> AMSEAYNWKSVVTGAGGGFVPGIIFNQSEPDLIYARTDIGGAYRWNQATGSWVSISDAVGWVDWNKNGVDALATDPVDPDKVYMATGTYTNSWDDNGQIMRSGDRGNTWQSTPLPFKVGGNMPGRSAGERLVIDPNKNSILFFGARSGNGLWKSTDSGVTWSKVSSFPNVGTYIQNPTLEYGNDLVGLSWITFDPNTGTPGNATQTIYVGVADTASSVYRSTDGGATWTAIPGQPTGYLPHHGVLSSTGDLYITYSNGVGPYDGSKGEVWKLNTASGAWTNISPSAGTDNWYGFGGLAVDAQHPDTVMVSSLNAWWPDEVIFRSTNGGATWSRIWDWGSYPERSYKFAMDITAAPWLNHGVTNSTSLDPSPKLGWMMGDLEIDPFNSNRMMYGTGATIYGTNNLTSWDTGGKVNIAVMAKGVEETAVLGLISPPSGTAHLITALGDVSGFRYEDLTQAPVKFQTSPSWATTTGIDFAELNPSYVVRVGG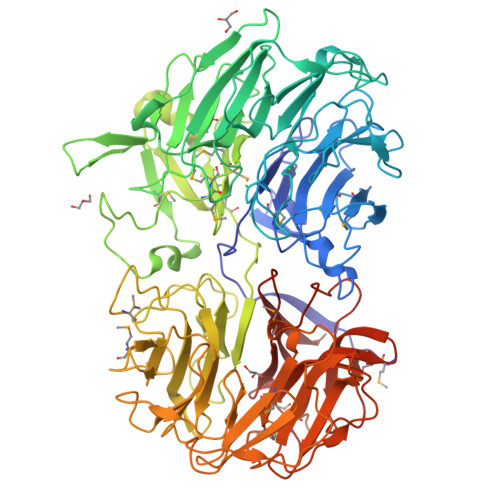ADKEKDPGMKSIGISNDGGVNWYMPNSEPSSGTKTTAGQGQVAVSASGNSILWSTSDLGVYYSKTTGNSWTVSAGVPAGAKVASDRVNPNKFYAFYAGIFYVSTDGGATFTATAAAGLPANNVGGLQPNQAQISMKAMPGIEGDVWFAGGNTVENKYGLWHSINSGTSFTKLTNVEEADLIGFGMAAPGQNYMALYTVARMDGVRGVFRSDDAGASWVRINDDAHQYAKINMAITGDPRVYGRVYLGTNGRGTLYADPV> CGCGAA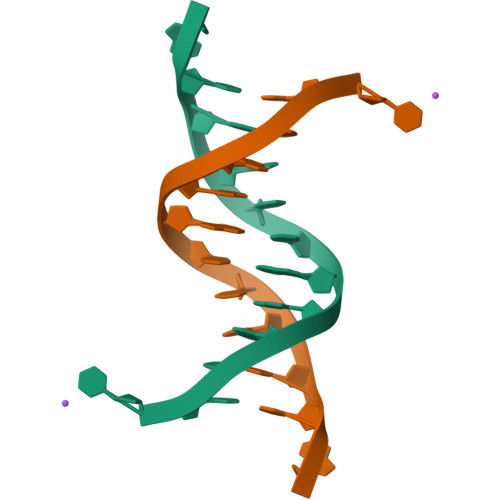TTXGCG> GSHMAKTYDYLFKLLLIGDSGVGKTCVLFRFSEDAFNSTFISTIGIDFKIRTIELDGKRIKLQIWDTAGLERFRTITTAYYRGAMGIMLVYDITNEKSFDNIRNWIRNIEEHASADVEKMILGNKCDVNDKRQVSKERGEKLA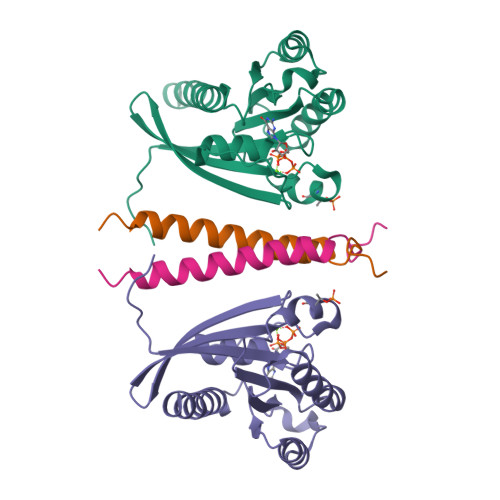LDYGIKFMETSAKANINVENAFFTLARDIKAKMDKKLEGNS;> GSHMGPNKMVVDLTDPNRPRFTLQELRDVLQERNKLKSQLLVVQEELQCYKSG>RKPKTGILMLNMGGPETLGDVHDFLLRLFLDQDLMTLPIQNKLAPFIAKRLTPKIQEQYRRIGGGSPIKIWTSKQGEGMVKLLDELSPNTAPHKYYIGFRYVHPLTEEAIEEMERDGLERAIAFTQYPQYSCSTTGSSLNAIYRYYNQVGRKPTMKWSTIDRWPTHHLLIQCFADHILKELDHFPLEKRSEVVILFSAHSLPMSVVNRGDPYPQEVSATVQKVMERLEYCNPYRLVWQSKVGPMPWLGPQTDESIKGLCERGRKNILLVPIAFTSDCIETLYELDIEYSQVLAKECGVENIRRAESLNGNPLFSKALADLVHSHIQSNELCSKQLTLSCPLCVNPVCRETKSFFTSQ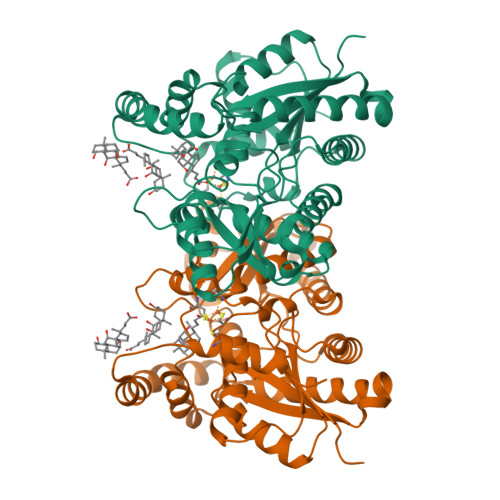QL[2x]>[2x]MGSDKIHHHHHHKDLLGREVEIPSNVNRIVAVGPGALRLIAYLKATDMVVGVEDFEKLRPYGRPYILAYPELKKLPSVGPGGPGKLPDLESLITLQPDVVFITYVDRKTAKDIQE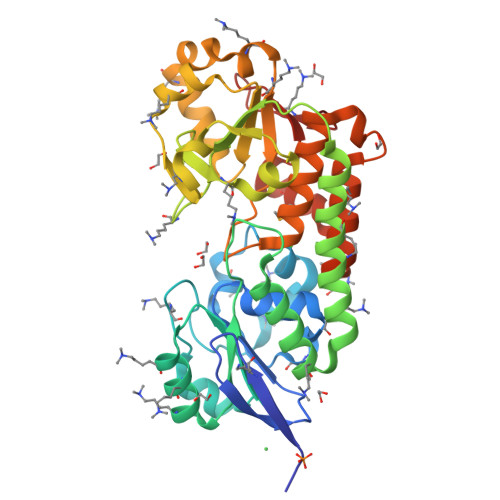KTGIPVVVLSYGNLGTFEDEDLFRSIELAGKILGREERAHEVVDFIRKAQEDLVTRSEGVESPTVYVGGIGYKGAHGIDSTEAKYPPFVVLHARNVVDELGEGHKFIDPEKLLVWNPEYIFIDENGLSLVLDDYSKHREFYESLSAVKRGKVYGILPYNYYTTNIGTALADAYFIGKVLYPERFTDIDPEEKADEIYEFLLGKRVYGEMAEQFGGFGKIDLPSGRILRGTW>MTVEHAQLTSNDLLVKSISSSPSPSPWDFLGRVLQFQHGDHKRWWD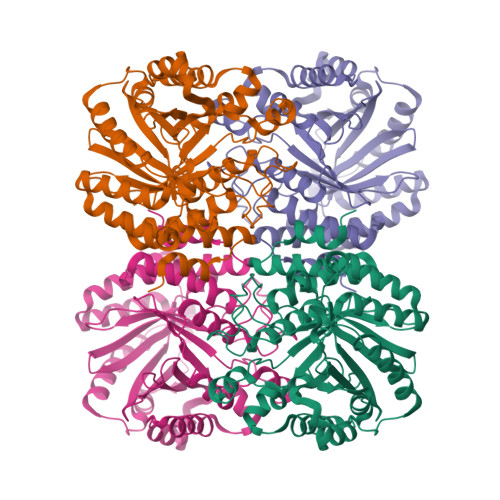VLAPVFGISMASIGYKLDVQYRHLLVLYDAVIPNMGPFPNSNASNITWTSPFPPGPLEASVNYQAGESSMFRFTIEPVGPHAGTPADPVNELAAKQLMQRLGQLQPGGVDSTMFDHFYPLLCVDGPEARRQWDSIAHIYHKCHTVTALDMQRSAACTLKTYFPPLLRSTIMNTSMVDIMFDAVESFRKQSGLYFDYTKIKEFMSEEKTHETMMVDRSYLSFDCLDPAKSRIKIYTEAKVKTLEEAYSFWSLGGRLSGPEIDYGFKIVSQMWDAIYSKELPGGKQRENNHIQINWEMSAKDSSVAPKLYLTVIEDYDAYVSSAIVDLFTGLGWAAHVQTHKKIEKEAYPMCDANPQSTHAYVWISLAYKKTGPYITVYTNPGASILEKA[4x]> MRVLVTGGSGYIGSHTCVQLLQNGHDVIILDNLCNSKRSVLPVIERLGGKHPTFVEGDIRNEALMTEILHDHAIDTVIHFAGLKAVGESVQKPLEYYDNNVNGTLRLISAMRAANVKNFIFSSVATVYGDNPKIPYVESFPTGTPQSPYGKSKLMVEQILTDLQKAQPDWSIALLRYFNPVGAHPSGDMGEDPQGIPNNLMPYIAQVAVGRRDSLAIFGNDYPTEDGTGVRDYIHVMDLADGHVVAMEKLANKPGVHIYNLGAGVGNSVLDVVNAFSKACGKPVNYHFAPRRE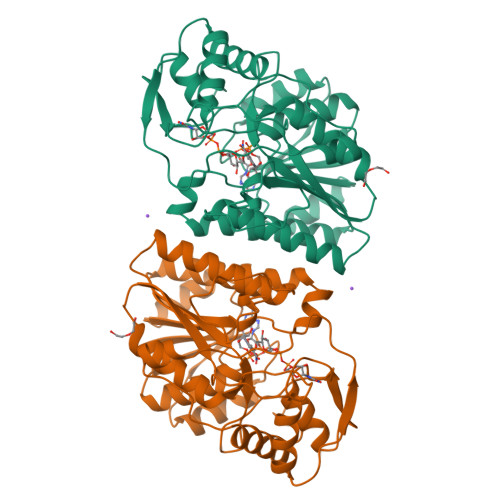GDLPAYWADASKADRELNWRVTRTLDEMAQDTWHWQSRHPQGYPD> PQAGSLDLQIDEEQPAGTLIGDISAGLPAGTAAPLMYFISAQEGSGVGTDLAIDEHSGVVRTARVLDREQRDRYRFTAVTPDGATVEVTVRVADINDHAPAFPQARAALQVPEHTAFGTRYPLEPARDADAGRLGTQGYALSGDGAGETFRLETRPGPDGTPVPELVVTGELDRENRSHYMLQLEAYDGGSPPRRAQALLDVTLLDINDHAPAFNQSRYHAVVSESLAPGSPVLQVFASDADAGVNGAVTYEINRRQSEGDGPFSIDAHTGLLQLERPLDFEQRRVHELVVQARDGGAHPELGSAFVTVHVRDANDNQPSMTVIFLSADGSPQVSEAAP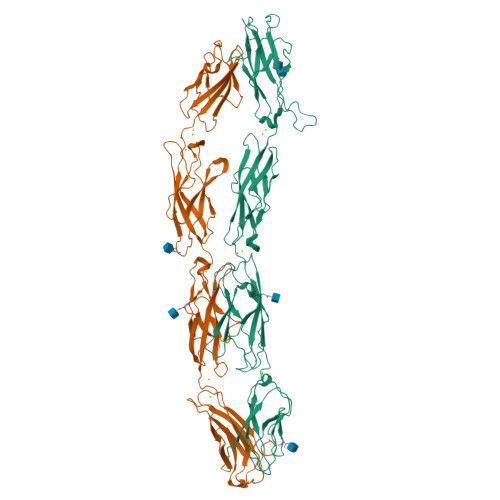PGQLVARISVSDPDDGDFAHVNVSLEGGEGHFALSTQDSVIYLVCVARRLDREERDAYNLRVTATDSGSPPLRAEAAFVLHV;> MDLAPDRATGRPWLPLHTLSVSQLLRVFWLLSLLPGQAWVHGAEPRQVFQVLEEQPPGTLVGTIQTRPGFTYRLSESHALFAINSSTGALYTTSTIDRESLPSDVINLVVLSSAPTYPTEVRVLVRDLNDNAPVFPDPSIVVTFKEDSSSGRQVILDTATDSDIGSNGVDHRSYRIIRGNEAGRFRLDITLNPSGEGAFLHLVSKGGLDREVTPQYQLLVEVEDKGEPKRRGYLQVNVTVQDINDNPPVFGSSHYQAGVPEDAVVGSSVLQVAAADADEGTNADIRYRLQDEGTPFQMDPETGLITVREPLDFEARRQYSLTVQAMDRGVPSLTGRAEALIQLLDVNDNDPVVKFRYFPATSRYASVDENAQVGTVVALLTVTDADSPAANGNISVQILGGNEQRHFEVQSSKVPNLSLIKVASALDRERIPSYNLTVSVSDNYGAPPGAAVQARSSVASLVIFVND>MDASTLGSFTGGQLRRLGSVAGLSRADVETYAQVLTDALGPVAQRPLSLAPPTRTFLSDDHTPVEFSLSFRPGAAPAMRVLVEPGCGATSLADNGRAGLEAVRTMARRWHFTTDALDELLDLFLPPAPQG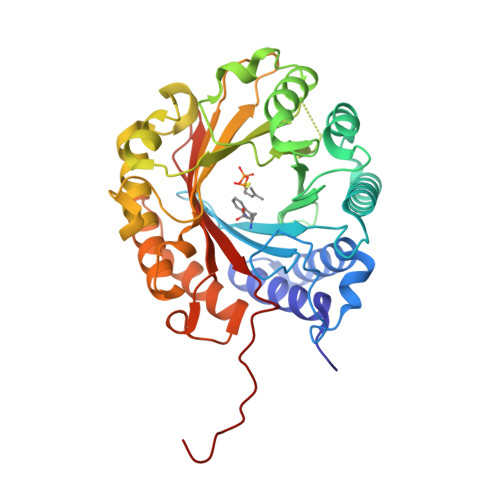PLALWCALELRPGGVPGVKVYLNPAVGGEERSAATVREALRRLGHHQAFDSLPQGSGYPFLALDLGNWTEPRAKVYLRHDNLTAGRAARLSRTDSGLVPTAVEGFFRTAAGPGSDAGGLDGRPAQSCHSFTDPGAERPSGFTLYIPVRDYVRHDGEALARASTVLHHHGMDASVLHRALAALTERRPEDGVGLIAYLALAGQRDQPPRVTAYLSSEAYTVRPPVVELVPR[2x]> 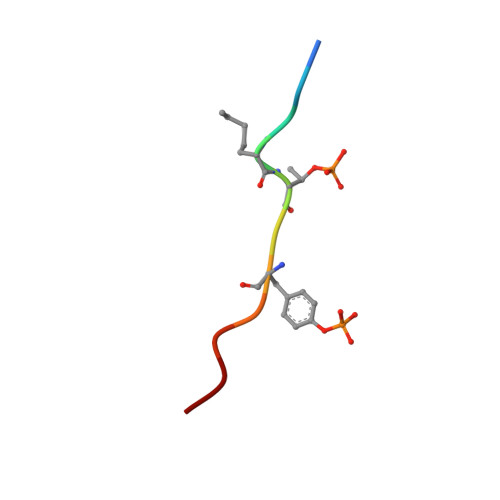DDEATGYVATR N-{cis-3-[methyl(7H-pyrrolo[2,3-d]pyrimidin-4-yl)amino]cyclobutyl}propane-1-sulfonamide | C14 H21 N5 O2 S | 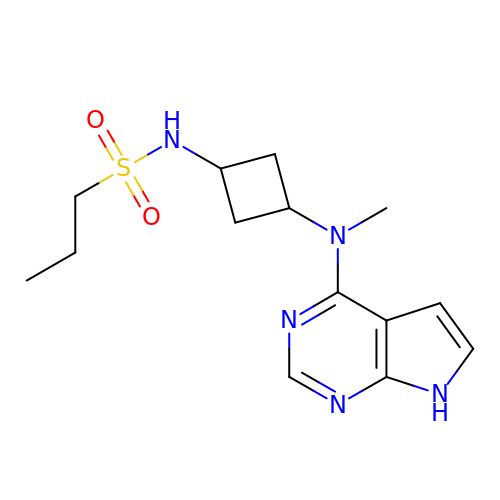IUEWXNHSKRWHDY-PHIMTYICSA-N>[2x]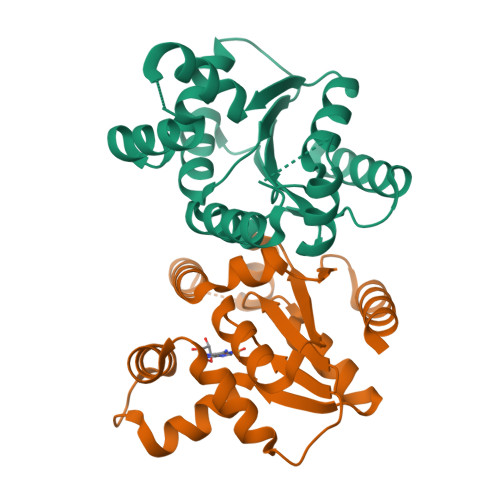IKVILITGMPGSGKSEFAKLLKERGAKVIVMSDVVRKRYSIEAKPGERLMDFAKRLREIYGDGVVARLCVEELGTSNHDLVVFDGVRSLAEVEEFKRLLGDSVYIVAVHSPPKIRYKRMIERLRSDDSKEISELIRRDREELKLGIGEVIAMADYIITNDSNYEEFKRRCEEVTDRVLK> VAPTLTARLYSLLFRRTSTFALTIVVGALLFERAFDQGADAIYEHI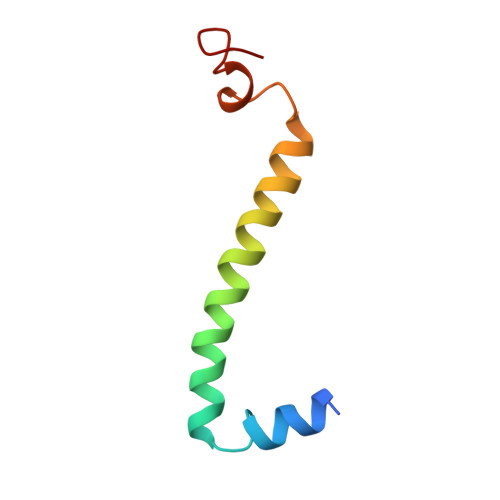NEGKLWKHIKHKYENK> MSWSHPQFEKGAMTLSTIRWDVDIIAQSSIVHRDDYTSVGSDTFTLFRREKIIGPDGQILQIPLISGSSFRGVLRRVGEALTAEVLGYEDVALPVPAAHLLTNGGRLAKSAHPLTDEEERNLKELLPQIAVFGGAASGRVMSGLLSVSKVLP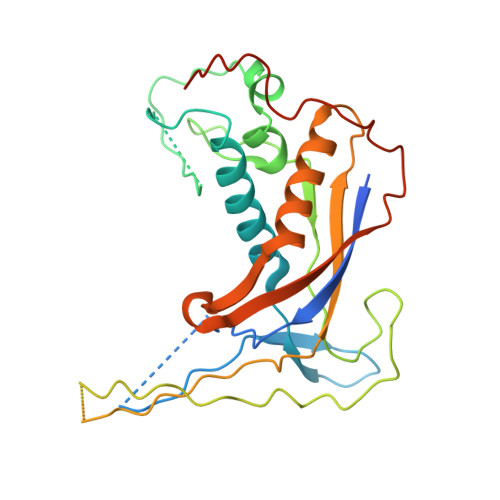EIAELAHLLPRPPHSTPLLPAVLSVADESFTHLPDHRPSTGGAPRTDHADGSPLGRFAIETLPAGTRLQTWARLDNATEHQAAFFDNVLSTFAAHGHLGGRSAAGHGQVTATVTATALRGSLPRPTVDWVNQLADDRDAAIAALTRLT> MSLTKVSSLGYPRLGENREWKKLIEAYWAGKVSKNDLFAGAKELRLDFLKKQLNAGLDLIPVGDFSLYDHILDLSVQFNIIPKRFAKEPIDIDLYFAIARGNKENVASSMKKWFNTNYHYIVPEWSKQRPKLNNNRLLDLYLEAREVVGDKAKPVITGPITYVALSTGVEDFTAAVKSLLPLYKQVFTELVKAGASYIQVDEPIFVTDEGKDYLQAAKAVYAYFAKEVPDAKFIFQTYFEGLIDSQVLSQLPVDAFGLDFVYGLEENLEAIKTGAFKGKEIFAGVIDGRNIWSSDFVKTSALLETIEEQSAALTIQPSCSLLHVPVTTKNETDLDPVLRNGLAFADEKLTEVKRLAEHLDGREDPAYDLHIAHFDALQAADFRNVKLEDLSRVATKRPSDFAKRRDIQQEKLHLPLLPTTTIGSFPQSREIRRTRLAW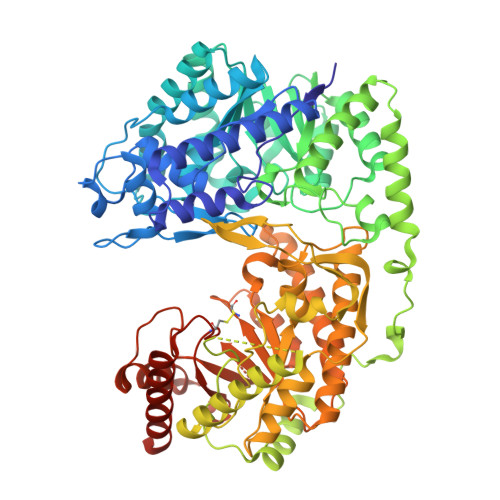KRGDISDAEYKQFIQAEIERWIRIQEDLDLDVLVHGEFERVDMVEFFGQKLAGFTTTKFGWVQSYGSRAVKPPIIYGDVQHLEPITVEETVYAQSLTDRPVKGMLTGPITITNWSFERTDIPRDQLFNQIGLAIKDEIKLLENAGIAIIQVDEAALREGLPLRKSKQKAYLDDAVHAFHIATSSVKDETQIHTHMCYSKFDEIIDAIRALDADVISIETSRSHGDIIESFETAVYPLGIGLGVYDIHSPRVPTKEEVVANIERPLRQLSPTQFWVNPDCGLKTRQEPETIAALKVLVAATKEVRQKLGNEGHHHHHH6-ethoxy-6-oxohexanoic acid | C8 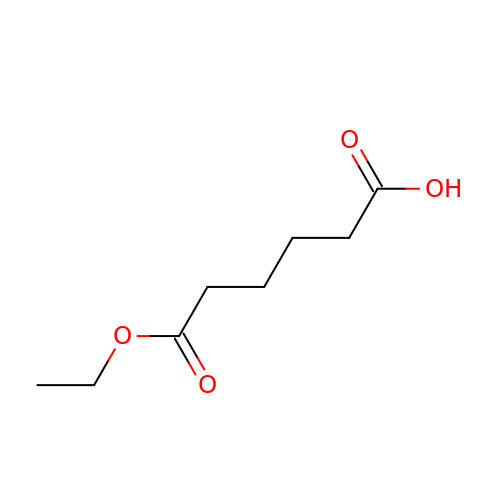H14 O4 | UZNLHJCCGYKCIL-UHFFFAOYSA-N>MHNHNHNHNHNHNGGENLYFQGASLTEIEHLVQSVCKSYRETCQLRLEDLLRQRSNIFSREEVTGYQRKSMWEMWERCAHHLTEAIQYVVEFAKRLSGFMELCQNDQIVLLKAGAMEVVLVRMCRAYNADNRTVFFEGKYGGMELFRALG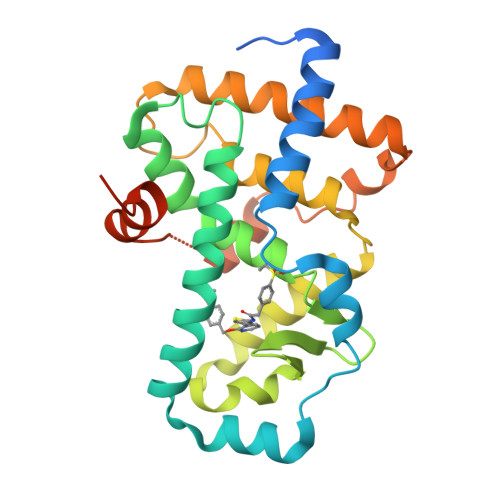CSELISSIFDFSHSLSALHFSEDEIALYTALVLINAHRPGLQEKRKVEQLQYNLELAFHHHLCKTHRQSILAKLPPKGKLRSLCSQHVERLQIFQHLHPIVVQAAFPPLYKELFS[2x]> STDNAETGVIEAGNTDTDFSGELAAPGSNHTNVKFLFDRSRLLNVIKVLEKDAVFPRPFPTQEGAQQDDGYFCLLTPRPTVASRPATRFGLYANPSGSGVLANTSLDFNFYSLACFTYFRSDLEVTVVSLEPDLEFAVGWFPSGSEYQASSFVYDQLHVPFHFTGRTPRAFASKGGKVSFVLPWNSVSSVLPVRWGGASKLSSATRGLPAHADWGTIYAFVPRPNEKKSTAVKHVAVYIRYKNARAWCPSMLPFRSYK;> DRVTTQTAGNTAINTQSSLGVLCAYVEDPTKSDPPSSSTDQPTTTFTAIDRWYTGRLNSWTKAVKTFSFQAVPLPGAFLSRQGGLNGGAFTATLHRHFLMKCGWQVQVQCNLTQFHQGALLVAMVPETTLDVKPDGKAKSLQELNEEQWVEMSDDYRTGKNMPFQSLGTYYRPPNWTWGPNFINPYQVTVFPHQILNARTSTSVDINVPYIGETPTQSSETQNSWTLLVMVLVPLDYKEGATTDPEITFSVRPTSPYFNGLRNRYTA;> PIPTAPRENSLMFLSTLPDDTVPAYGNVRTPPVNYLPGEITDLLQLARIPTLMAFERVPEPVPASDTYVPYVAVPTQFDDRPLISFPITLSDPVYQNTLVGAISSNFANYRGCIQITLTFCGPMMARGKFLLSYSPPNGTQPQTLSEAMQCTYSIWDIGLNSSWTFVVPYISPSDYRETRAITNSVYSADGWFSLHKLTKITLPPDCPQSPCILFFASAGEDYTLRLPVDCNP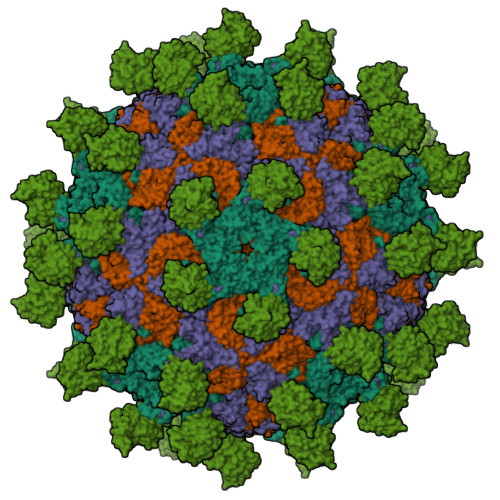SYVF;> RGNNGNMTFNYYANTYQNSVDFSTSSSASGAGPGNSRGGLAGLLTNFSGILNPLGYLK;> SMACYGGFDLYFILDKSGSVLHHWNEIYYFVEQLAHKFISPQLRMSFIVFSTRGTTLMKLTEDREQIRQGLEELQKVLPGGDTYMHEGFERASEQIYYENRQGYRTASVIIALTDGELHEDLFFYSEREANRSRDLGAIVYAVGVKDFNETQLARIADSKDHVFPVNDGFQALQGIIHSILKKSC>[2x]MRGSHHHHHHGSDSELISENMHTKLYMEGTVNG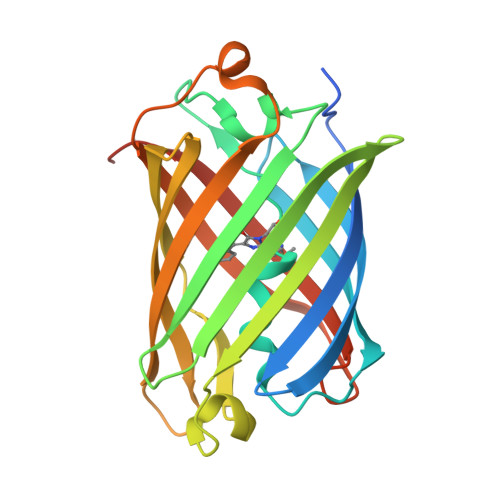HHFKCTSEGEGKPYEGTQTCKIKVVEGGPLPFAFDILATSFMYGSKTFINHTQGIPDFFKQSFPEGFTWERITTYEDGGVLTATQDTSLQNGCLIYNVKINGVNFPSNGPVMQKKTLGWEANTEMLYPADSGLRGHNQMALKLVGGGYLHCSLKTTYRSKKPAKNLKMPGFYFVDRKLERIKEADKETYVEQHEMAVARYCDLPSKLGHS>AQDMVSPPPPIADEPLTVNTGIYLIESYSLDDKAETFKVNAFLSLSWKDRRLAFDPVRSGVRVKTYEPEAIWIPEIRFVNVENARDADVVDISVSPDGTVQYLERFSARVLSPLDFRRYPFDSQTLHIYLIVRSVDTRNIVLAVDLEKVGKNDDVFLTGWDIESFTAVVKPANFALEDRLESKLDYQLRISRQYFSYIPNIILPMLFILFISWTAFWSTSYEANVTLVVSTLIAHIAFNILVCTNLPKTPYMTYTGAIIFMIYLFYFVAVIEV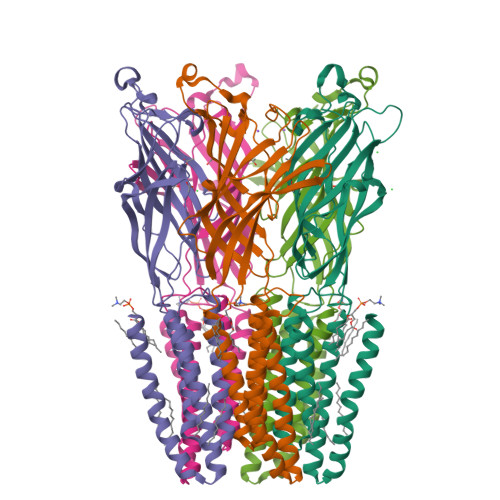TVQHYLKVESQPARAASITRASRIAFPVVFLLANIILAFLFFGF[5x]>[2x]GAMDDSSLQKVELQTDVYMVCLQHALSTENFEVMGLLIGNFACGIAKISAVIILRRLDKKKDRVEISSEQLLKAAAEAERLTVELNRPMRVLGWYHSHPHITVCPSHVDVRTQATYQTMDHSFVGLIFSVFSEGKESKEHEIFLNCFQSDNGEATEIPLEIVHTPDISDRCLRTMTDLSKILVQEEEDMAEACKDHPDVLASIHNNAVRTRALIHITDIITKPLVQT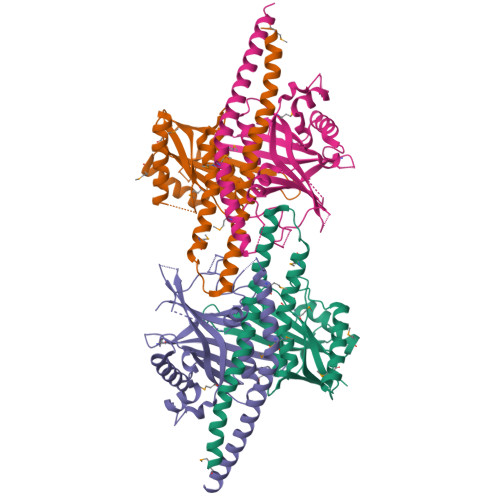FEKRIALNKLRATHLQRQLQELQKMCNG;>[2x]MADSDLLVTISGAALSLLFFENVRSVGNQMGFLLGEALEFIVKTYTDSDNQVETVKIHINVEAIVTCPLADLLHDSTNHINKEKLKDFVRDKSKQVIGWFCFRRNTTNLTLTLKDKLLHKQFASHFSGVNGCKEDFFLTCLLNASTSETSGTHKFRHVFLRHNKRGMFEPISLKINNLGDDASRHDGSDYKPTPVRKSTRTPDSFTKLIESLNLDVARIDGLDSAMLIQKAAEHHLMSLIPKVCESDLEVAELEKQVHELKIKIATQQLAKRLKINGENCDRISKASKD We report the 2.3-Å resolution crystal structure of QDE-1, a cRdRP from Neurospora crassa, and find that it forms a relatively compact dimeric molecule, each subunit of which comprises several domains with, at its core, a catalytic apparatus and protein fold strikingly similar to the catalytic core of the DNA-dependent RNA polymerases responsible for transcription. A cell-encoded RNA-dependent RNA polymerase (cRdRP) is also involved, in plants, fungi, protozoa, and certain animals, but apparently not insects and vertebrates, producing dsRNA triggers and hence amplifying the PTGS response. The polypeptide chain then leads into a “catalytic” domain (residues 647–807; 914–1,161) that houses the three proposed catalytic aspartic acid residues (D1007, D1009, and D1011) within an active site cleft formed between two DPBB subdomains (DPBB1, residues 690–792, and DPBB2, residues 916–1,018). Overall, QDE-1 exists as a compact, but flexible, dimeric enzyme with metal binding sites confirming positions of the catalytic sites but with extensive additional structure whose biological functions are less immediately clear.

The structure of QDE-1 ΔN was initially solved by multiwavelength anomalous diffraction (MAD) analysis of a crystal of selenomethionated protein, expressed in yeast, to a resolution of 3.2 Å. The structure was then refined against a higher resolution dataset extending to 2.3 Å. These crystals belong to space group P21, and the crystallographic asymmetric unit contains two subunits, which together form a compact pyramidal object with dimensions of 90 × 70 × 127 Å3. The two constituent subunits are related by an approximate 2-fold axis and are in such intimate contact (over 2,000 Å2 of contact area per subunit) that we would expect this to represent a functional dimer. QDE-1 ΔN has 1,026 residues, and the final model contains 933 residues in subunit A and 930 residues in subunit B (residues are missing from the N- and C-termini and from some flexible loops). The refined structure at 2.3 Å has an Rwork of 21.7% (Rfree = 26.4%), and the stereochemistry is good (root mean square deviation [rmsd] bond = 0.013 Å, rmsd angle = 1.9°, 2.3% of residues are in disallowed regions of the Ramachandran plot; Table 1). The proposed dsRNA product binding channels are not identical in the two subunits, because the disposition of the domains is different: subunit A has a “closed” conformation, with the head and slab clamped down on the active site cleft, whereas an 11° rotation of the head and 2° rotation of the slab render the B subunit more open and provide space for an RNA duplex. Analysis of electron density maps showed a Mg2+ ion coordinated by these aspartic acid side chains (the functional significance of this is underscored by the observation that the QDE-1 polymerase activity is dependent on divalent cations).

>ESARSQVQVHAPVVAARLRNIWPKFPKWLHEAPLAVAWEVTRLFMHCKVDLEDESLGLKYDPSWSTARDVTDIWKTLYRLDAFRGKPFPEKPPNDVFVTAMTGNFESKGSAVVLSAVLDYNPDNSPTAPLYLVKLKPLMFEQGCRLTRRFGPDRFFEILIPSPTSTSPSVPPVVSKQPAAVEEVIQWLTMGQHSLVGRQWRAFFAKDAGYRKPLREFQLRAEDPKPIIKERVHFFAETGITFRPDVFKTRSVVPAEEPVEQRTEFKVSQMLDWLLQLDNNTWQPHLKLFSRIQLGLSKTYAIMTLEPHQIRHHKTDLLSPSGTGEVMNDGVGRMSRSVAKRIRDVLGLGDVPSAVQGRFGSAKGMWVIDVDDTGDEDWIETYPSQRKWECDFVDKHQRTLEVRSVASELKSAGLNLQLLPVLEDRARDKVKMRQAIGDRLINDLQRQFSEQKHALNRPVEFRQWVYESYSSRATRVSHGRVPFLAGLPDSQEETLNFLMNSGFDPKKQKYLQDIAWDLQKRKCDTLKSKLNIRVGRSAYIYMIADFWGVLEENEVHVGFSSKFRDEEESFTLLSDCDVLVARSPAHFPSDIQRVRAVFKPELHSLKDVIIFSTKGDVPLAKKLSGGDYDGDMAWVCWDPEIVDGFVNAEMPLEPDLSRYLKKDKTTFKQLMASHGTGSAAKEQTTYDMIQKSFHFALQPNFLGMCTNYKERLCYINNSVSNKPAIILSSLVGNLVDQSKQGIVFNEASWAQLRRELLGGALSLPDPMYKSDSWLGRGEPTHIIDYLKFSIARPAIDKELEAFHNAMKAAKDTEDGAHFWDPDLASYYTFFKEISDKSRSSALLFTTLKNRIGEVEKEYGRLVKNKEMRDSKDPYPVRVNQVYEKWCAITPEAMDKSGANYDSKVIRLLELSFLADREMNTWALLRASTAFKLYYHKSPKFVWQMAGRQLAYIKAQMTSRPGEGAPALMTAFMYAGLMPDKKFTKQYVARLEGDGSEYPDPEVYEVLGDDDFDGIGFTGNGDY[2x]> MDESQPRK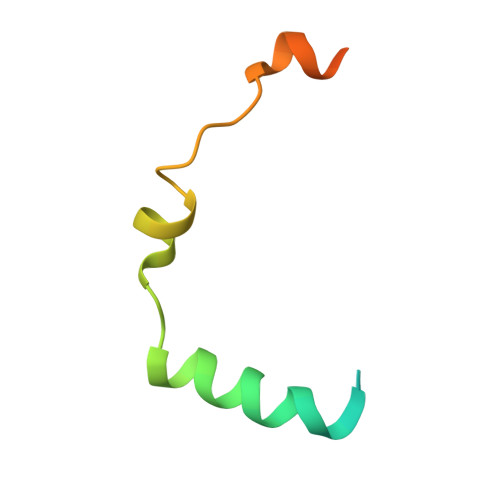PIPAWASGNLLTQAIRQQYYKPIDVDRMYGTIDSPKLEELFNKSKPRYFKR>MRIQHNIAALNTHRNLAANNAAASKNLEKLSSGFKINRAGDDAAGLAISEKMRGQISGLNMASKNSSDAISLIQTAEGGLNETHAILQRMRELAVQSRNDTNDEATNDRSNLNDELKQLQEEITRISSQMEFNNKKLLDGSQSTNGLTFQIGANAGQTITMKISTMSATKLGVDAAKASISKGTAASKAIKSIDDAINTVSKTRSALGAVQNRLEHTINNLGTSAENLTA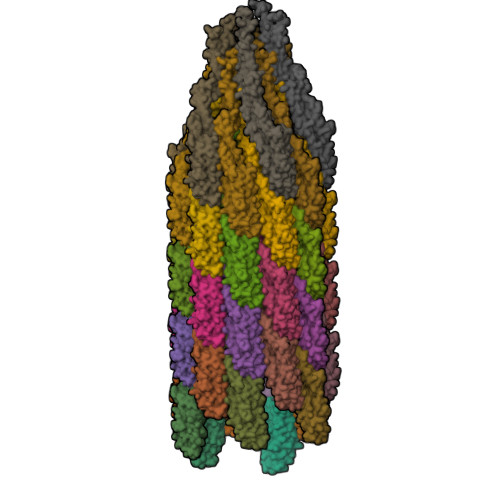AESRIRDTDMAAEMMAFTKNNILTQAAQSMLAQANQQPQGVLQLLQ[44x]> MIVNVIQKDRLKEQKLQFIRNHQQAFDVEPIYPLPLFEDFVTSIEGDCSLEASCKIESDKLIASRFLLFFEDKTQEWQKYLHQSLTFFGLVE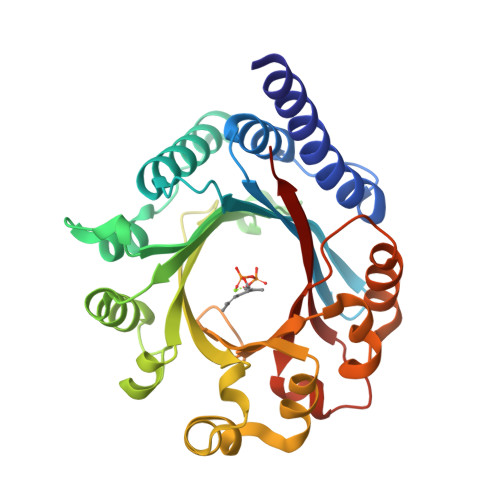NRVGVKINYSLLQQFLGSSFDFSKVTVLSAGIDLRNNLAESSLKMHIRIKDYPEKLDKAFALSDGAADGNYLKDFVNLIGFDFYFNGKSEIEIYAEVQEDDFFKPEINNLVWQHFPKTALQPLKASSLFATGLSKANNNPVLYYHLKNRQDLTNYFKLNDTAQRVHSFYQHQDILPYMWVGTAQKELEKTRIENIRLYYYKSFKMESN>MSSELLLLTSDRDCEAVLPALGLLPHRVRVLPPEPGAILSAGTHDVVLVDARTDLAGARDLCRVLAVGDAPVLAVVNEGGLVTVSAEWGVDDILLPTAGPAEIDARLRLLTTRRGADAGEGDGMLTVGDLVIEESTYTARLKGRALELTYKEFELLK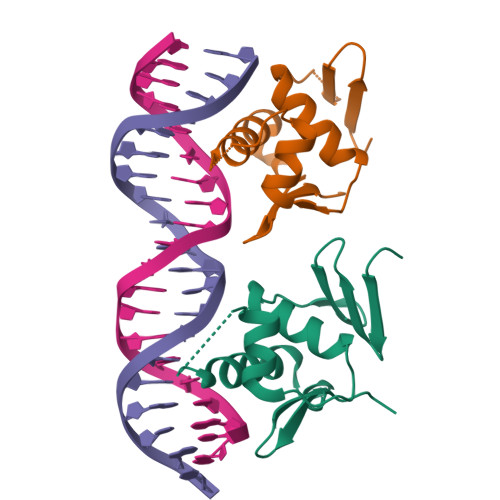YLAQHAGRVFTRAQLLQEVWGYDFFGGTRTVDVHVRRLRAKLGPEYDSMIGTVRNVGYKFVRPSRSSQPASPIVAEERQDAATQADAPAQRSAESAVVR[2x]> TEAAAQPHALPADAPDIAPERDLLSKFDGLIAERQKLLDSGVTDPFAIVMEQVKSPTEAVIRGKDTILLGTYNYMGMTFDPDVIAAGKEALEKFGSGTYGSRMLNGTFHDHMEVEQALRDFYGTTGAIVFSTGYMANLGIISTLAGKGEYVILDADSHASIYDGCQQGNAEIVRFRHNSVEDLDKRLGRLPKEPAKLVVLEGVYSMLGDIAPLKEMVAVAKKHGAMVLVDEAHSMGFFGPNGRGVYEAQGLEGQIDFVVGTFSKSVGTVGGFVVSNHPKFEAVRLACRPYIFTASLPPSVVATATTSIRKL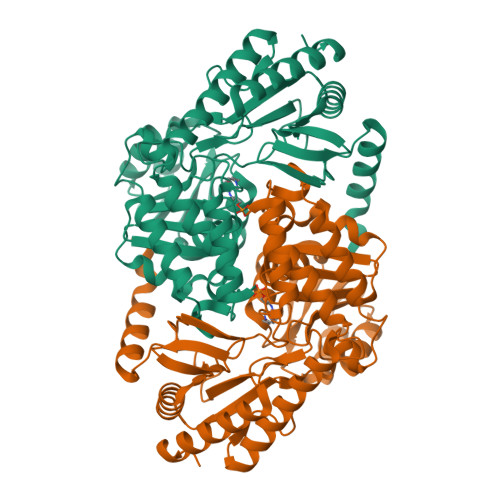MTAHEKRERLWSNARALHGGLKAMGFRLGTETCDSAIVAVMLEDQEQAAMMWQALLDGGLYVNMARPPATPAGTFLLRCSICAEHTPAQIQTVLGMFQAAGRAVGVIGLEHHHHHH>[2x]GAMAPVPVTKLV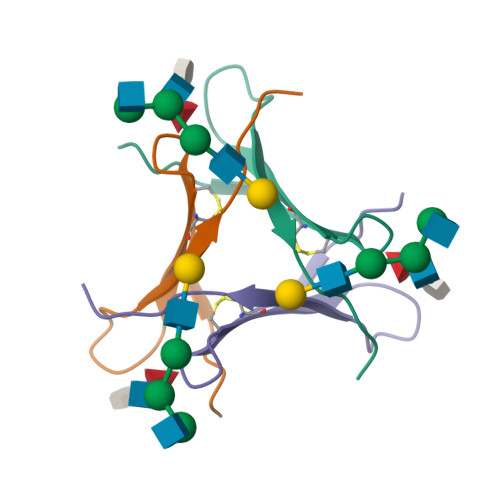CDGDTYKCTAYLDFGDGRWVAQWDTNVFHTG> GSMVEATAQETDRPRFSFSIAAREGKARTGTIEMKRGVIRTPAFMPVGTAATVKALKPETVRATGADIILGNTYHLMLRPGAERIAKLGGLHSFMGWDRPILTDSGGYQVMSLSSLTKQ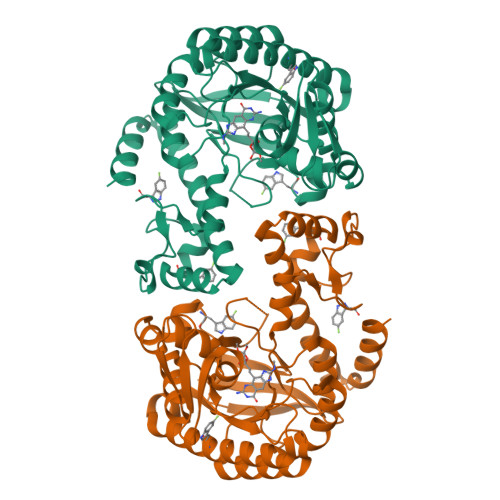SEEGVTFKSHLDGSRHMLSPERSIEIQHLLGSDIVMAFDECTPYPATPSRAASSMERSMRWAKRSRDAFDSRKEQAENAALFGIQQGSVFENLRQQSADALAEIGFDGYAVGGLAVGEGQDEMFRVLDFSVPMLPDDKPHYLMGVGKPDDIVGAVERGIDMFDCVLPTRSGRNGQAFTWDGPINIRNARFSEDLKPLDSECHCAVCQKWSRAYIHHLIRAGEILGAMLMTEHNIAFYQQLMQKIRDSISEGRFSQFAQDFRARYFARNS>GSSHHHHHHSSSHMKILVIQGPNLNMLGHRDPRLYGMVTLDQIHEIMQTFVKQGNLDVELEFFQTNFEGEIIDKIQESVGSDYEGIIINPGAFSHTSIAIADAIMLAGKPVIEVHLTNIQAREEFRKNSYTGAACGGVIMGFGPLGYNMALMAMVNILAEMKAF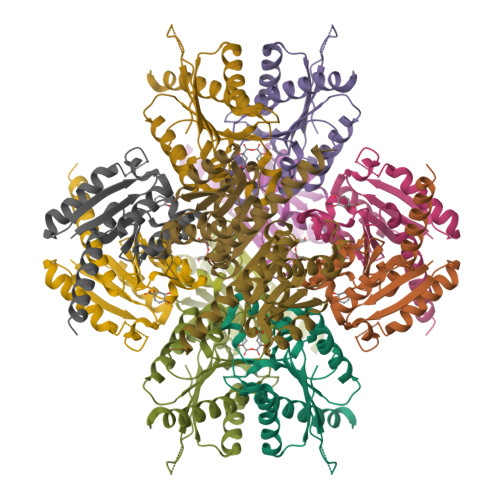QEAQKNNPNNPINNQK[12x]>[2x]GAMDPDLEATLRAIVHSATSLVDARYGAMEVHDRQHRVL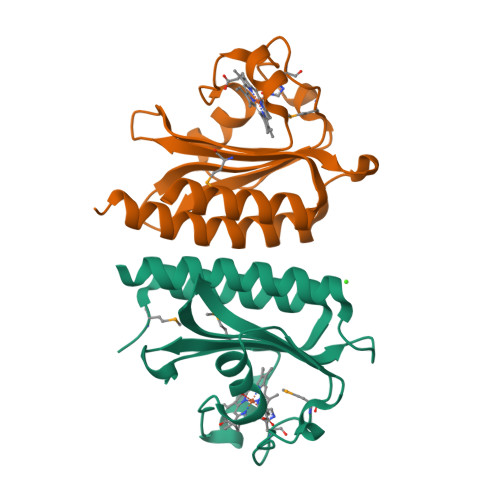HFVYEGIDEETVRRIGHLPKGLGVIGLLIEDPKPLRLDDVSAHPASIGFPPYHPPMRTFLGVPVRVRDESFGTLYLTDKTNGQPFSDDDEVLVQALAAAAGIAVANARLYQQAK> AHHHHHHPGGPGSENLYFQGGSSGIDVN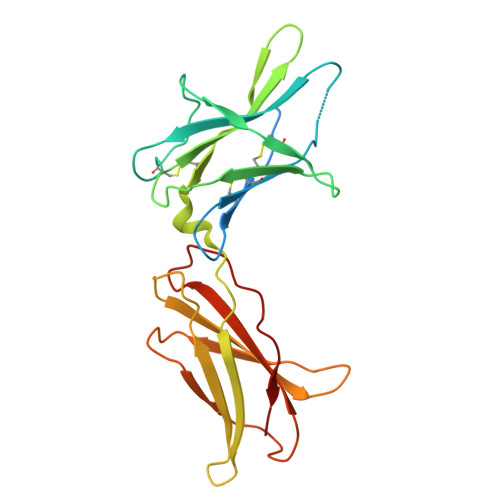INISCETDGYLTKMTCRWSTSTIQSLAESTLQLRYHRSSLYCSDIPSIHPISEPKDCYLQSDGFYECIFQPIFLLSGYTMWIRIQHSLGSLDSPPTCVLPDSVVKPLPPSSVKAEITINIGLLKISWEKPVFPENNLQFQIRYGLSGKEVQWKMYEVYDAKSKSVSLPVPDLSAVYAVQVRCKRLDGLGYWSNWSNPAYTVVMD> GSHMNGLIYAVGGYDGNTHLNSVEAYDPERNEWSLVAPLSTRRSGVGVAVLNGLIYAVGGYDGNTHLNSVEAYDPERNEWSLVAPLSTRRSGVGVAVLNGLIYAVGGYDGN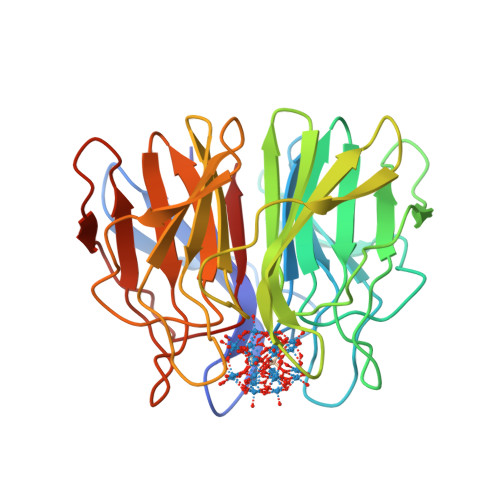THLNSVEAYDPERNEWSLVAPLSTRRSGVGVAVLNGLIYAVGGYDGNTHLNSVEAYDPERNEWSLVAPLSTRRSGVGVAVLNGLIYAVGGYDGNTHLNSVEAYDPERNEWSLVAPLSTRRSGVGVAVLNGLIYAVGGYDGNTHLNSVEAYDPERNEWSLVAPLSTRRSGVGVAVL> SHENAATLNDVKTLVQQLYTTLCIEQHQLNKERELIERLEDLKEQLAPLEKVRIEISRKAEKRTTLVLWGGLAYMATQFGIL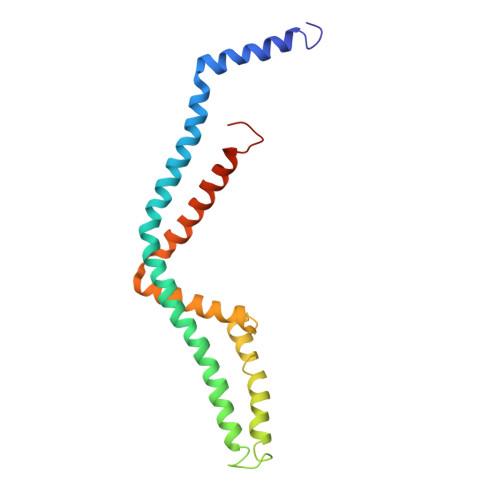ARLTWWEYSWDIMEPVTYFITYGSAMAMYAYFVMTRQEYVYPEARDRQYLLFFHKGAKKSRFDLEKYNQLKDAIAQAEMDLKRLRDPLQVHLPLRQ>[2x]QAENPIFTDVFTADPAALVHKGRVYLYAGRDEAPDNTTFFVMNEWLVYSSDDMANWEAHGPGLRAKDFTWAKG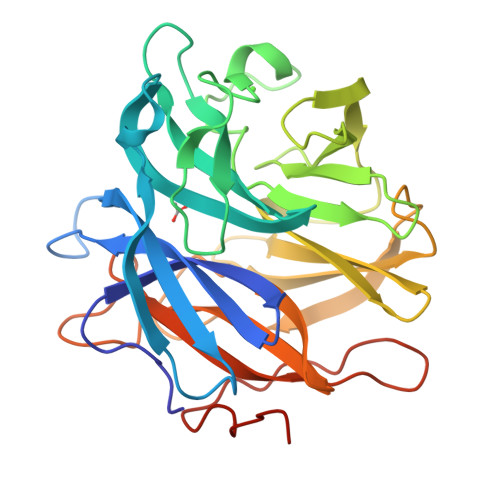DAWASQVIERNGKFYWYVTVRHDDTKPGFAIGVAVGDSPIGPFKDALGKALITNDMTTDTPIDWDDIDPSVFIDDDGQAYLFWGNTRPRYAKLKKNMVELDGPIRAIEGLPEFTEAIWVHKYQDNYYLSYAMGFPEKIGYAMGKSIKGPWVYKGILNEVAGNTPTNHQAIIEFNNKHYFIYHTGAGRPDGGQYRRSVSIDELFYNPDGTIKRIVMTTEGVAPNKSPERVKKAAK(4R)-4-methyl-7-[(1R)-1-phenylethoxy]-1,3,4,5-tetrahydro-2H-1,5-benzodiazepin-2-one | C18 H20 N2 O2 | 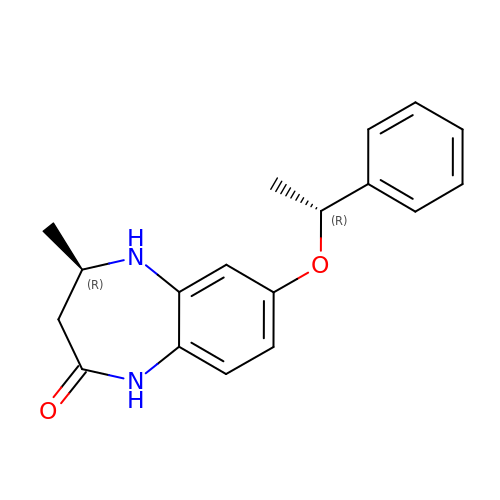ORPRVEZBBPKRRY-CHWSQXEVSA-N Here, we study the kinetics and substrate specificity of an AldDH enzyme from the Clostridium phytofermentans fucose/rhamnose utilisation BMC, Cphy1178. The overall structure corresponds to other members in the aldehyde dehydrogenase family, with a catalytic domain (residues 238–427, highlighted pink), a cofactor-binding domain with the Rossman-fold type nucleotide binding architecture (residues 28–108, 127–237, and 428–447, highlighted grey), and an oligomerisation domain (residues 109–126 and 448–462, highlighted green). The catalytic and nucleotide binding domains come together to form an extended nucleotide and ligand-binding tunnel that is open at both ends, with the catalytic cysteine (C269) at the centre of the tunnel and the NAD+ cofactor binding at one side. Cphy1178 forms a tetrameric quaternary structure generated by crystal symmetry, with molecules related by D2 symmetry.

The structures of Cphy1178 were also solved with mutations in active site residues, C269A with bound CoA (1.77 Å resolution) and H387A (2.08 Å resolution) to ensure that mutation of these residues did not destabilise the structure of the protein. The structure of Cphy117820–462(C269A) was determined using crystals soaked with 10 mM CoA. The cofactor showed good electron density for the adenosine group, but poor density for the pantothenic acid group, particularly the terminal region with the sulphydryl group in the active site, which has no visible electron density. While there is clear electron density for the nucleotide and phosphate-proximal portion of the pantothenate group of the CoA, the β-mercapto ethylamine group is not visible, indicating that the distal arm of CoA is flexible in the absence of thio-acyl substrates bound to the catalytic cysteine for acyl transfer. The adenine ring is flipped by 180 degrees relative to its position in the NAD+ structure and makes hydrogen-bonding contacts with both the side chain and carbonyl oxygen of Asparagine 160, and the carbonyl oxygen of Threonine 134, placing the phospho-ribose group above both of the nucleotide binding pockets. The phosphate groups between the nucleotide and pantothenate group are held in place by hydrogen bonds formed between the side-chain nitrogen atoms of Histidine 162 and Arginine 318. A comparison of the structure of the NAD+ and CoA bound forms of the protein show that the structures are essentially identical, with an rmsd Cα of 0.24 Å over 431 residues. The two structures differ only in the position of the loop between residues 215 and 223, where P219, G220 and V221 are shifted toward the adenine ring in the NAD+-bound structure. In contrast to the models of CoA binding to the Pseudomonas DmpF aldehyde dehydrogenase36 and Lactobacillus reuteri PduP aldehyde dehydrogenase25 our crystal structure shows distinct adenine-binding modes for NAD+ and CoA.

> MGQLTQTNKTELGVFDDMNQAIEAAKEAQLVVKKMSMDQREKIISAIRKKTIEHAETLARMAVEETGMGNVGHKILKHQLVAEKTPGTEDITTTAWSGDRGLTLVEMGPFGVIGAITPCTNPSETIICNTIGMLAGGNTVVFNPHPAAIKTSNFAVQLINEASLSAGGPVNIACSVRKPTLDSSKIMMSHQDIPLIAATGGPGVVTAVLQSGKRGIGAGAGNPPVLVDETADIRKAAEDIINGCTFDNNLPAIAEKEVVAIDAIANELMNYMVKEQGCYAITKEQQEKLTNLVITPKGLNRNCVGKDARTLLGMIGIDVPSNIRCIIFEGEKEHPLISEELMMPILGIVRAKSFDDAVEKAVWLEHGNRHSAHIHSKNVDRITTYAKAIDTAILVKNAPSYAAIGFGGEGFCTFTIASRTGEGLTSASTFTKRRRCVMSDSLCIR>HVTQSSSAITPGQTAELYPGDIKSVLLTAEQIQARIAELGEQIGNDYRELSATTGQDLLLITVLKGAVLFVTDLARAIPVPTQFEFMAVSSYGSSTSSSGVVRILKDLDRDIHGRDVLIVEDV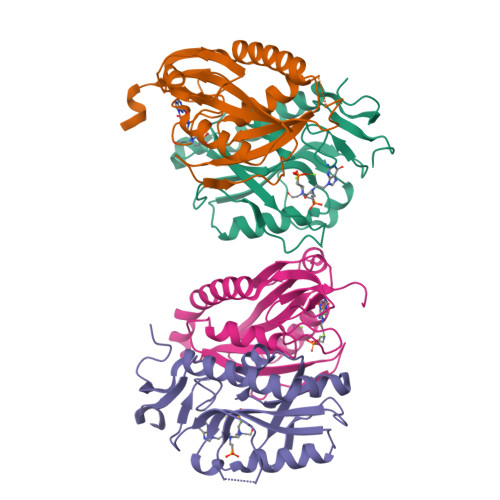VDSGLTLSWLSRNLTSRNPRSLRVCTLLRKPDAVHANVEIAYVGFDIPNDFVVGYGLDYDERYRDLSYIGTLDPRVYQ[4x]>[2x]MGSSHHHHHHSQDPNSMDPLAVSAASVVSMSNDVLKPETPKGPII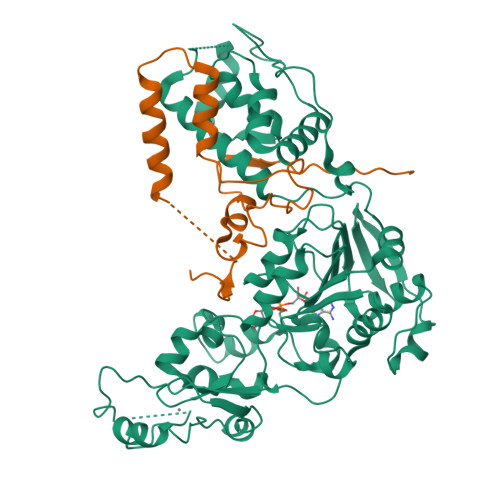ISKNPSNGIFYGPSFTKRESLNARMFLKYYGAHKFLDTYLPEDLNSLYIYYLIKLLGFEVKDQALIGTINSIVHINSQERVQDLGSAISVTNVEDPLAKKQTVRLIKDLQRAINKVLCTRLRLSNFFTIDHFIQKLHTARKILVLTGAGVSTSLGIPDFRSSEGFYSKIKHLGLDDPQDVFNYNIFMHDPSVFYNIANMVLPPEKIYSPLHSFIKMLQMKGKLLRNYTQNIDNLESYAGISTDKLVQCHGSFATATCVTCHWNLPGERIFNKIRNLELPLCPYCYKKRREYFPEGYNNKVGVAASQGSMSERPPYILNSYGVLKPDITFFGEALPNKFHKSIREDILECDLLICIGTSLKVAPVSEIVNMVPSHVPQVLINRDPVKHAEFDLSLLGYCDDIAAMVAQKCGWTIPHKKWNDLKNKNFKSQEKDKGVYVVTSDEHPKTL;>[2x]GSMNTIITHPGKMELVYVSDSDDSSSDNDSLTDLESLSSGESNEIKVTNDLDTSAEKDQIQAGKWFDPVLDWRKSDRELTKNILWRIADKTTYDKETITDLIEQGIPKHSYLSGNPLTSVTNDICSVENYETSSAFFYQQVHKKDRLQYLPLYAVSTFE> MASLLTETMPFRMTM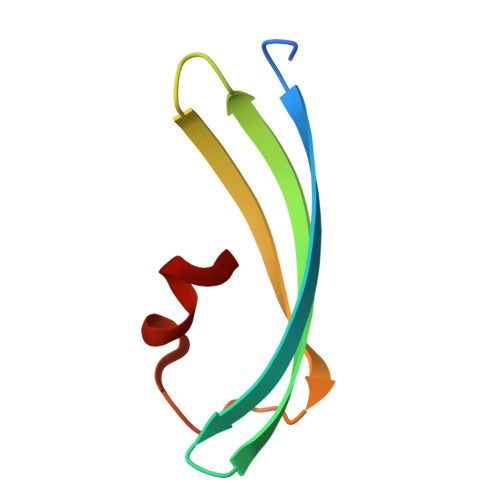EGTVNGHHFKCTGKGEGNPFEGTQDMKIEVIEGGPLPFAFDILSTSC> ATIKDVAKRANVSTTTVSHVINKTRFVAEETRNAVWAAIKELHYSPSAVARSLKVNHTKSIGLLATSSEAAYFAEIIEAVEKNCFQKGYTLILGNAWNNLEKQRAYLSMMAQKRVDGLLVMCSEYPEPLLAMLEEYRHIPMVVMDRGEAKADFTDAVIDNAFEGGYMAGRYLIERGHREIGVIPGPLERNTGAGRLAGFMKAME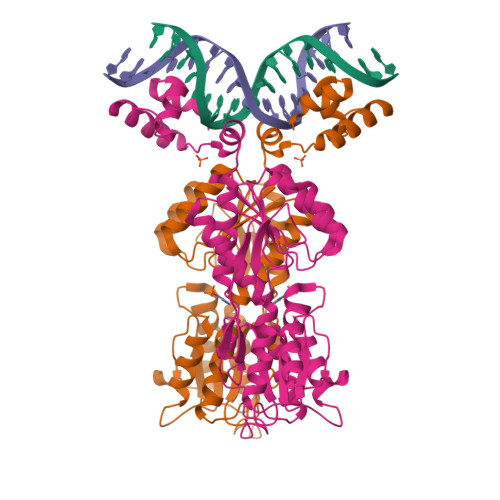EAMIKVPESWIVQGDFEPESGYRAMQQILSQPHRPTAVFCGGDIMAMGALCAADEMGLRVPQDVSLIGYDNVRNARYFTPALTTIHQPKDSLGETAFNMLLDRIVNKREEPQSIEVHPRLIERRSVADGPFRDYRR>[3x]MSEKKAVIGVVTISDRASKGIYEDISGKAIIDYLKDVIITPFEVEYRVIPDERDLIEKTLIELADEKGCSLILTTGGTGPAPRDVTPEATEAVC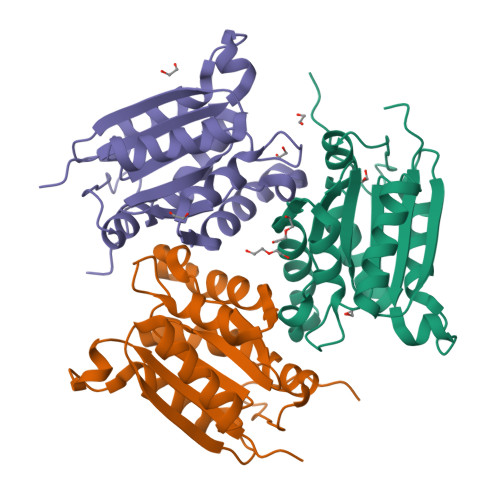EKMLPGFGELMRQVSLKQVPTAILSRQTAGIRGSCLIVNLPGKPQSIKVCLDAVMPAIPYCIDLIGGAYIDTDPNKVKAFRPKK> HHHHHHMANLPILLDYWPSMFGMRARVALREKGVEFEYREEDFSNKSPLLLQSNPIHKKIPVLVHNGKPVCESLNVVQYVDEAWPEKNPFFPSDPYGRAQARFWADFVDKKFTDAQFKVWGKKGEEQEAGKKEFIEAVKILESELGDKPYFGGDSFGYVDISLITFSSWFQAYEKFGNFSIESESPKLIAWAKRCMEKESVSKS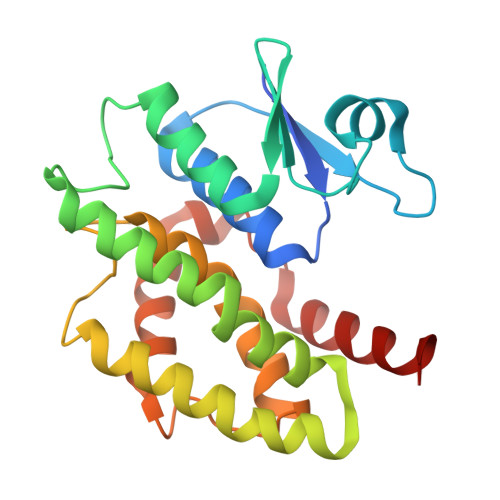LPDSEKIVAYAAEYRKNNL2-[(5R,7S)-6-HYDROXY-2-PHENYLADAMANTAN-2-YL]-1-(3-HYDROXYAZETIDIN-1-YL)ETHAN-1-ONE | C21 H27 N O3 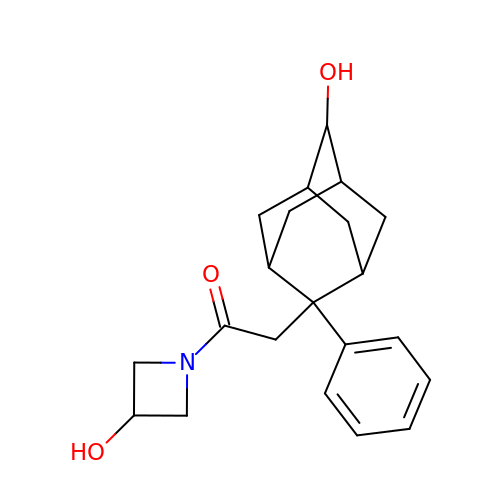| OAAZMUGLOXGVNH-TUOVGCFYSA-N> SAELASEAGVQQQPLELRPGEYRVLLCVDIGETRGGGHRPELLRELQRLHVTHTVRKLHVGDFVWVAQETNPRDPANPGELVLDHIVERKRLDDLCSSIIDGRFREQKFRLKRCGLERRVYLVEEHGSVHNLSLPESTLLQAVTNTQVIDGFFVKRTADIKESAAYLALLTRGLQRLYQGHTLRSRPWGTPGNPESGAMTSPNPLCSLLTFSDFNAGAIKNKAQSVREVFARQLMQVRGVSGEKAAALVDRYSTPASLLAAYDACATPKEQETLLSTIKCGRLQRNLGPALSRTLSQ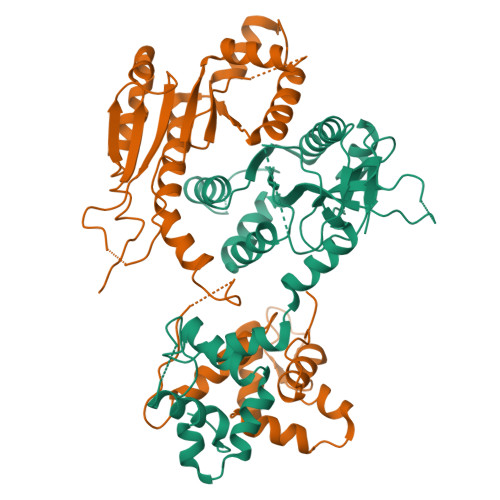LYCSYGPLT;> MARVGPGRAGVSCQGRGRGRGGSGQRRPPTWEISDSDAEDSAGSEAAARARDPAGERRAAAEALRLLRPEQVLKRLAVCVDTAILEDAGADVLMEALEALGCECRIEPQRPARSLRWTRASPDPCPRSLPPEVWAAGEQELLLLLEPEEFLQGVATLTQISGPTHWVPWISPETTARPHLAVIGLDAYLWSRQHVSRGTQQPESPKVAGAEVAVSWPEVEEALVLLQLWANLDVLLVASWQELSRHVCAVTKALAQYPLKQYRESQAFSFCTAGRWAAGEPVARDGAGLQAAWRRQIRQFSRVSPAVADAVVTAFPSPRLLQQALEACSTERERMGLLADLPVPPSEGGRPRRVGPDLSRRICLFLTTANPDLLLDLGS> MVPISPIETVPVKLKPGMDGPKVKQWPLTEEKIKALVEICTEMEKEGKISKIGPENPYNTPVFAIKKKDSTKWRKLVDFRELNKRTQDFWEVQLGIPHPAGLKKKKSVTVLDVGDAYFSVPLDEDFRKYTAFTIPSINNETPGIRYQYNVLPQGWKGSPAIFQSSMTKILEPFAAQNPDIVIYQYMDDLYVGSDLEIGQHRTKIEELRQHLLRWGLTTPDKKHQKEPPFLWMGYELHPDKWTVQPIVLPEKDSWTVNDIQKLVGKLNWASQIYPGIKVRQLSKLLRGTKALTEVIPLTEEAELELAENREILKEPVHGVYYDPSKDLIAEIQKQGQGQWTYQIYQEPFKNLKTGKYARMRGAHTNDVKQLTEAVQKITTESIVIWGKTPKFKLPIQKETWETWWTEYWQATWIPEWEFVNTPPLVKLWYQLEKEPIVGAETFYVDGAANRETKLGKAGYVTNKGRQKVVPLTNTTNQKTELQAIYLALQDSGLEVNIVTDSQYALGIIQAQPDKSESELVNQIIEQLIKKEKVYLAWVPAHKGIGGNEQVDKLVSAG;> PISPIETVPVKLKPGMDGPKVKQWPLTEEKIKALVEICTEMEKEGKISKIGPENPYNTPVFAIKKKDSTKWRKLVDFRELNKRTQDFWEVQLGIPHPAGLKKKKSVTVLDVGDAYFSVPLDEDFRKYTAFTIPSINNKTPGIRYQYNVLPQGWKGSPAIFQSSMTKILEPFKKQNPDIVIYQYMDDLYVGSDLEIGQHRTKIEELRQHLLRWGLTTPDKKHQKEPPFLWMGYELHPDKWTVQPIVLPEKDSWTVNDIQKLVGKLNWASQIYPGIKVRQLSKLLRGTKALTEVIPLTEEAELELAENREILKEPVHGVYYDPSKDLIAEIQKQGQGQWTYQIYQEPFKNLKTGKYARMRGAHTNDVKQLTEAVQKITTESIVIWGKTPKFKLPIQKETWETWWTEYWQATWIPEWEFVNTPPLVKLWYQ

HIV-1 reverse transcriptase (RT) (hereinafter referred to as RT) plays an essential role in the viral life cycle by reverse transcribing the single-stranded RNA genome to a double-stranded DNA copy. There are two main types of RT inhibitors: nucleoside RT inhibitors (NRTIs), which act as chain terminators and compete with incoming nucleotides in the polymerase active site, and non-nucleoside RT inhibitors (NNRTIs), which inhibit the activity of RT noncompetitively. NNRTIs are a group of structurally diverse compounds that bind to the non-nucleoside inhibitor-binding pocket (NNIBP) located ~10 Å from the polymerase active site. NNIBP is a hydrophobic pocket that emerges only when NNRTIs bind and induce conformational rearrangements of the residues defining the pocket.

Compound K-5a2 features a thiophene[3,2-d]pyrimidine central ring, and replaces the cyanophenyl right wing of ETR with a more extended piperidine-linked benzenesulfonamide group, while keeping the 4-cyano-2,6-dimethylphenyl structure in the left wing of ETR. In patients who failed ETR- or RPV-based therapies, E138K/Q/R are among the most frequently occurred mutations identified in RT. In the case of E138K RT, since the mutation does not disrupt the hydrophobic interactions between the inhibitors’ central thiophene ring and residue 138, 25a and K-5a2 maintain almost the same binding poses in the NNIBP and similar buried areas with each of the residues along the pocket as in their complexes with WT RT. There is no structure available for E138K RT and K101P RT in complex with either ETR or RPV; however, the structures of these two RT mutants in complex with K-5a2 and 25a provide a structural basis to understand why the mutations can render ETR and RPV less effective. In the structure of WT RT/ETR complex, the amino substituent of the central pyrimidine ring forms a salt bridge with the carboxyl side chain of Glu138. Transplanting Lys138 from the structure of E138K RT/K-5a2 complex into this structure reveals a severe charge-charge repulsion between the amino group in ETR and the side chain of Lys138, which would destabilize the binding of the inhibitor.>[4x]GSHMLSYRHSFHAGNHADVLKHTVQSLIIESLKE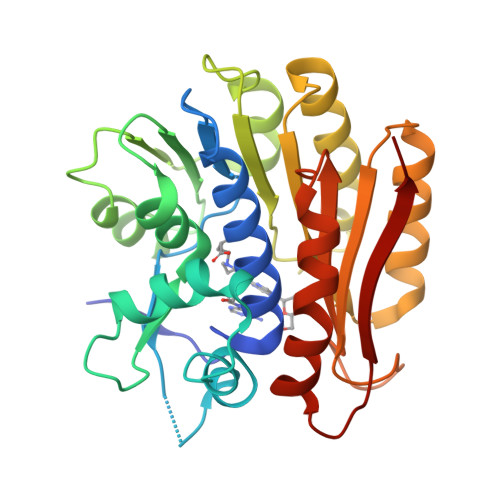KDKPFLYLDTHAGAGRYQLGSEHAERTGKYLEGIARIWQQDDLPAELEAYINVVKHFNRSGQLRYYPGSPLIARQLLREQDSLQLTELHPSDYPLLRSEFQKDSRARVEKADGFQQLKAKLPPVSRRGLILIDPPYEMKTDYQAVVSGIAEGYKRFATGTYALWYPVVLRQQIKRMIHDLEATGIRKILQIELAVLPDSDRRGMTASGMIVINPPWKLEQQMNNVLPWLHSKLVPAGTGHATVSWIVPE>GAMGSTSLEPTSTLVRVRKSAATLGIAIEGGANTRQPLPRIVTIQRGGSAHNCGQLKVGHVILEVNGQTLRGKEHKEAARIIAEAFKTKERDYIDFLVTEFNVML[6x];>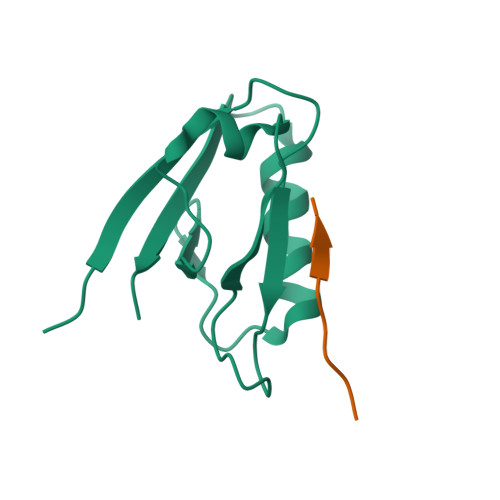PKEYDDELTFF[6x]> QPRPAFSAIRRNPPMGGNVVIFDTVITNQEEPYQNHSGRFVCTVPGYYYFTFQVLSQWEICLSIVSSSRGQVRRSLGFCD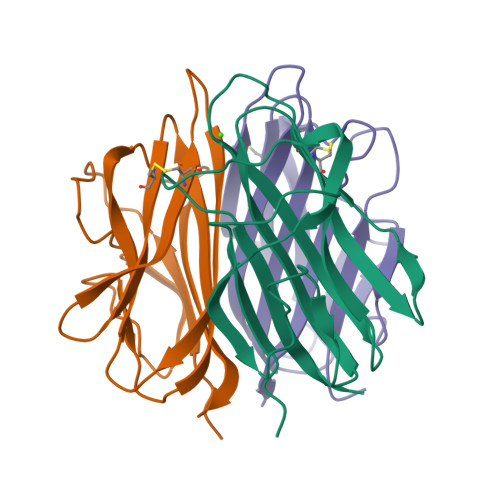TTNKGLFQVVSGGMVLQLQQGDQVWVEKDPKKGHIYQGSEADSVFSGFLIFPS;> TQKIAFSATRTINVPLRRDQTIRFDHVITNMNNNYEPRSGKFTCKVPGLYYFTYHASSRGNLCVNLMRGRERAQKVVTFCDYAYNTFQVTTGGMVLKLEQGENVFLQATDKNSLLGMEGANSIFSGFLLFPD;> KFQSVFTVTRQTHQPPAPNSLIRFNAVLTNPQGDYDTSTGKFTCKVPGLYYFVYHASHTANLCVLLYRSGVKVVTFCGHTSKTNQVNSGGVLLRLQVGEEVWLAVNDYYDMVGIQGSDSVFSGFLLFPD>GGSGVPGKVTLQKDAQNLIGISIGGGAQYCPGLYIVQVFDNTPAALDGTVAAGDEITGVNGRSIKGKTKVEVAKMIQEVKGEVTIHYNKLQADPKQLEVLFN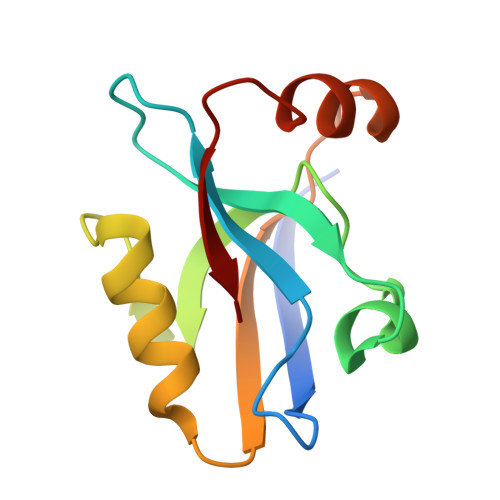GPGIESVKI[2x]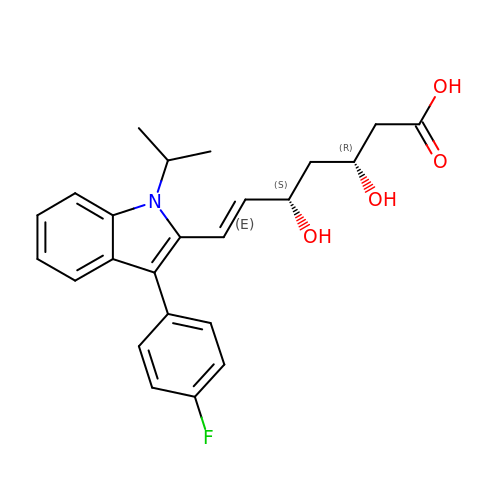(3R,5S,6E)-7-[3-(4-fluorophenyl)-1-(propan-2-yl)-1H-indol-2-yl]-3,5-dihydroxyhept-6-enoic acid | C24 H26 F N O4 | FJLGEFLZQAZZCD-MCBHFWOFSA-N> MITIPYLTAVSTYFSYGLLFAFGQLRDFFRRFIDWWFTSNLQGYAPICLGHEDFYIRRLYHRIQDCFERPISSAPDAWFDVVERYSNDNNKTLKRTTKTSRCLNLGSYNYLGFGSFDEYCTPRVIESLKKFSASTCSSRVDAGTTSVHAELEECVTRFVGKPAAVVFGMGYATNSAIIPVLIGKGGLIISDSLNHSSIVNGARGSGATIRVFQHNTPSHLERVLREQIAEGQPRTHRPWKKIIVVVEGIYSMEGEICHLPEVVAICKKYKAYVYLDEAHSIGAIGKTGKGICELLG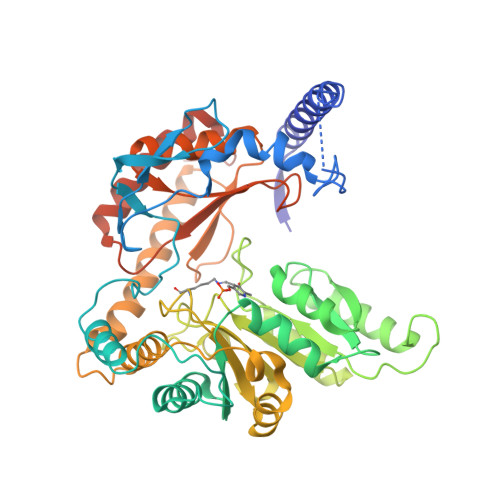VDTADVDVMMGTFTKSFGSCGGYIAGSKELIQYLKHQCPAHLYATSIPTPSAQQIISAIKVILGEDGSNRGAQKLARIRENSNFFRAELQKMGFEVLGDNDSPVMPIMLYNPAKIPAFSRECLRQKVAVVVVGFPATPLLLARARICISASHSREDLIRALKVISKVGDLSGIKYFPAEPKKIEQSKNDIKLD> ASAKADKKKAKEAAKAAKKKNKRAIRNSAKE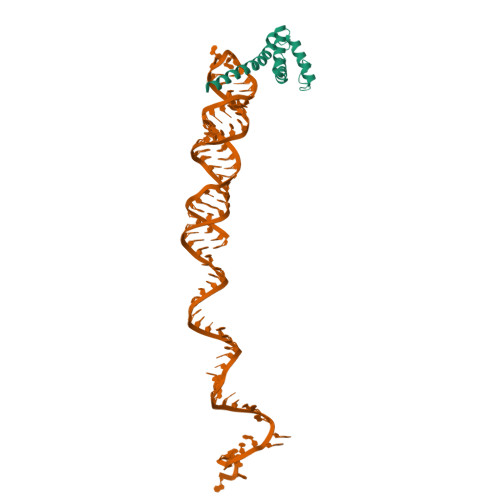ADYFGDADKATTIDEQVGLIVDSLNDEELVSTADKIKANAAGAKEVLKESAKTIVDSGKLPSSLLSYFV> MAYTTFSQTKNDQLKEPMFFGQPVNVARYDQQKYDIFEKLIEK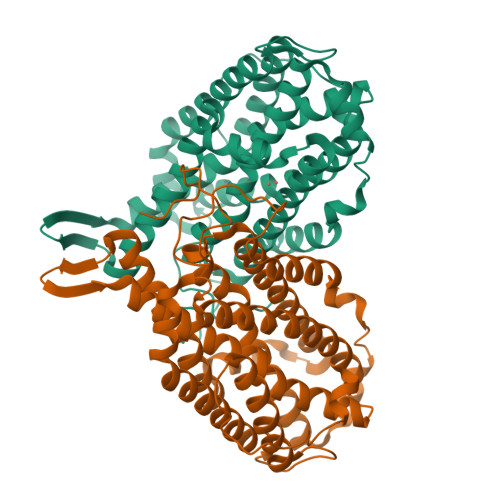QLSFFWRPEEVDVSRDRIDYQALPEHEKHIFISNLKYQTLLDSIQGRSPNVALLPLISIPELETWVETWAFSETIHSRSYTHIIRNIVNDPSVVFDDIVTNEQIQKRAEGISSYYDELIEMTSYWHLLGEGTHTVNGKTVTVSLRELKKKLYLCLMSVNALEAIRFYVSFACSFAFAERELMEGNAKIIRLIARDEALHLTGTQHMLNLLRSGADDPEMAEIAEECKQECYDLFVQAAQQEKDWADYLFRDGSMIGLNKDILCQYVEYITNIRMQAVGLDLPFQTRSNPIPWINTWLVSDNVQVAPQEVEVSSYLVGQIDSEVDTDDLSNFQL>MEKNFVITDPRLPDNPIIFASDGFLELTEYSREEILGRNARFLQGPETDQATVQKIRDAIRDQRETTVQLINYTKSGKKFWNLLHLQPVR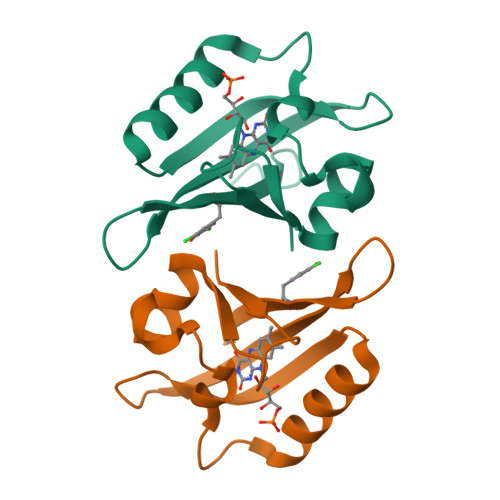DQKGELQYFXGVQLDGSDHVLEHHHHHH[2x]> GPMQDYTARAQVSEAILLAE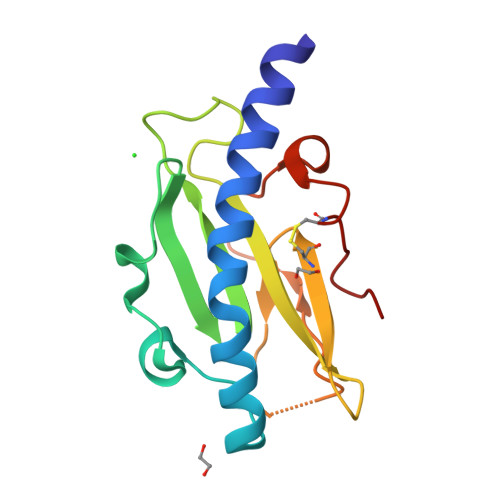GQKSAVTEYYLNHGEWPGNNTSAGVATSSEIKGKYVKSVEVKNGVVTAQMASSNVNNEIKGKKLSLWAKRQNGSVKWFCGQPVTRDKAKAANDDVTAAAAANGKKIDTKHLPSTCRDASDAS(1R)-6-HYDROXY-N-METHYL-N-[(1Z)-PROP-2-EN-1-YLIDENE]INDAN-1-AMINIUM 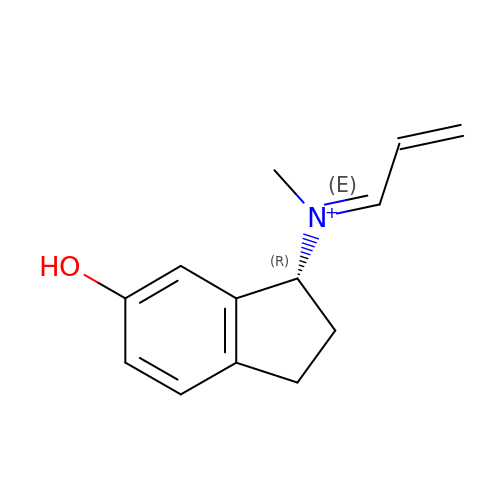| C13 H16 N O | ORDHHPNCLHHGNQ-SJWLEHQBSA-O>[6x]SNAMSQFMNLEGKVALVTGASRGIGKAIAELLAERGAKVIGTATSESGAQAISDYL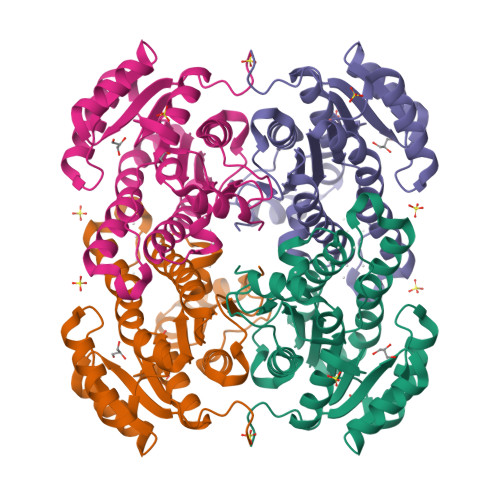GDNGKGMALNVTNPESIEAVLKAITDEFGGVDILVNNAGITRDNLLMRMKEEEWSDIMETNLTSIFRLSKAVLRGMMKKRQGRIINVGSVVGTMGNAGQANYAAAKAGVIGFTKSMAREVASRGVTVNTVAPGAIETDMTKALNDEQRTATLAQVPAGRLGDPREIASAVAFLASPEAAYITGETLHVNGGMYMI>MGKLLLILGSVIALPTFLAGGGDLDASDYTGVSFWLVTAALLASTVFFFVERDRVSAKWKTSLTVSGLVTGIAFWHYMYMRGVWIETGDSPTVFRYIDWLLTVPLLICEFYLILAAATNVAGSLFKKLLVGSLVMLVFGYMGEAGIMAAWPAFIIGCLAWVYMIYELWAGEGKSACNTASPAVQSAYNTMMYIIIFGWAIYPVGYFTGYLMGDGGSALNLNLIYNLADFVNKILFGLIIWNVAVKESSNAGHHHHH[6x]

Microbial ion-pumping rhodopsins (MRs) are extensively studied retinal-binding membrane proteins. The green-light absorbing proteorhodopsin (GPR) was originally discovered in marine γ-proteobacteria as the first bacterial rhodopsin and as an example of a new type of bacterial phototrophy. The bacterial green-light absorbing proton pump proteorhodopsin (GPR) has emerged as a model protein for MRs and is used here to address these open questions using cryo-electron microscopy (cryo-EM) and molecular dynamics (MD) simulations. GPR possesses an N-terminal signal sequence, akin to numerous membrane proteins, that is hypothesised to guide the correct insertion of the protein into the plasma membrane before subsequent proteolytic removal.

To this end, we expressed the GPR-A18L variant, introducing an alanine to leucine substitution (A18L) known to prevent cleavage of the signal peptide in the blue-light absorbing proteorhodopsin (BPR) when expressed in E. coli. Upon careful examination of the hexameric GPR map, two α-helical densities were identified in the central cavity, challenging the initially assumed C6 symmetry and revealing a C2 symmetry instead. In contrast, two α-helical densities were discovered filling the central cavity of the GPR-A18L hexamer, corresponding to the N-termini of protomers 1 and 4. Accommodation of additional signal peptides in the cavity is restricted due to their tilt of ~30° relative to the membrane normal. If two signal peptides occupy the space that will form the central cavity of the oligomer, this expands the diameter and thus permits the assembly of six protomers. The interfaces between protomers 1 and 4 are mainly formed by hydrophobic interactions where the signal peptides intersect and where they interact with TMH A of the opposing protomer. This includes a hydrogen bond formed between the two serine residues at position 10 and a salt bridge between K3 and D53 on TMH A. In total, these additional interactions, formed by the signal peptides with neighbouring protomers, account for an increased oligomerisation interface area compared to the pentamer of around 1400 Å2 (about 25% more), as calculated by PISA30. Interestingly, protomers 1 and 4 exhibit slight differences compared to the other protomers, likely due to the interaction of their signal peptides in the centre of the hexamer. This conformational change mainly affects the extracellular halves of TMHs E and F, and is also noticeable in the position of the retinal chromophore.Methionine sulfoxide reductase A (MsrA) is an important protein repair enzyme that specifically reduces methionine-S-sulfoxide to methionine. The Clostridium MsrA (CoMsrA), consisting of 209 residues, is classified into a 1-Cys type MsrA as it has a selenocysteine (Sec) residue at the catalytic site but contains no Cys residues. The CoMsrA structure folds into a common catalytic domain (residues 1–144) and a distinct helical domain (residues 145–209) which is absent from other known MsrA structures. The monomeric CoMsrA dimerizes in the presence of its substrate methionine sulfoxide via an intermolecular disulfide bond between catalytic Cys16 residues.

Dimeric CoMsrA was purified after substrate treatment to determine its crystal structure. The asymmetric unit contained one dimer and one monomer comprised of 204 residues (residues 5–208). The monomer in the asymmetric unit makes a dimer with a symmetric molecule. The area of the dimer interface was 1160 Å2 per monomer, corresponding to approximately 11% of the monomer’s surface area. The two catalytic domains from the pair of monomers face each other around the two catalytic Cys16 residues and occupy most of the dimer interface, whereas the helical domain lies distant from the interface. Interestingly, a central cavity is present in the surface model of the dimer, with a diameter of ~9 Å and a depth of ~12 Å. The two Cys16 residues constitute the base of the hole. However, although the two Cys16 residues were located close to each other in the dimeric MsrA structure within the asymmetric unit, no disulfide bond was observed. Thus, we speculate that the disulfide bond would be cleaved by intense synchrotron radiation. Interestingly, the active site pocket no longer exists in the dimeric MsrA with significant changes in the conformation of L1 and L2 loops.

>[3x]MDTNQKLSIAVFALGCFWGPDAQFGSIKGVVSTRVGYAGGTTNNPSYYNLGDHSESIEIQYDANVITYGELLNIFWNLHNPVYETTNRQYMSRIFYLDDGQKSEALEMKRQIEAANGEKIYTEIVPLENFYLAEGYHQKYYLQNTTKLYQTLKAIYGGFGNLVRSTLAARMNGYIAGNLSIASLKEEMDLVELPEDQYEKVLSIVEEIK>[4x]SGGGMLTLIQGKK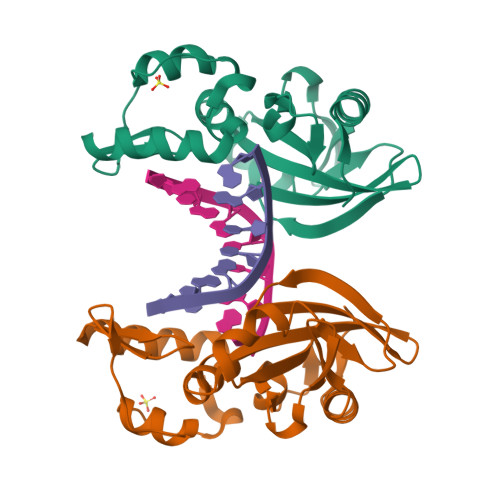IVNHLRSRLAFEYNGQLIKILSKNIVAVGSLRREEKMLNDVDLLIIVPEKKLLKHVLPNIRIKGLSFSVKVCGERKCVLFIEWEKKTYQLDLFTALAEEKPYAIFHFTGPVSYLIRIRAALKKKNYKLNQYGLFKNQTLVPLKITTEKELIKELGFTYRIPKKRL SAD efficiency studies were performed with the tetragonal form of thermolysin, a 316 residue protein with a predicted Bijvoet ratio of ∼1% for an X-ray wavelength of 1.54 Å. Here we investigate different cooling methods for several different protein crystals. We find that as long as ice formation is prevented and care is taken to limit damaging dehydration effects, gas stream cooling yields lower mosaicity than more rapid cooling methods (plunge cooling and hyperquenching). To assess the impact of the cooling method at the individual protein level, structures were determined of normal plunge cooled and gas stream cooled tetragonal thermolysin.

For gas stream cooling, we employed a vial mounting procedure to transfer the crystal directly to the cold gas stream rather than moving through the low-humidity ambient air. For the nine crystal/cryoprotectant combinations tested here, gas stream cooling at 100 K using the vial mounting approach yielded lower mosaicity than normal plunge cooling into liquid nitro­gen at 77 K. For the subset of crystals tested, the anomalous signal from gas stream cooling was comparable to or stronger than that from plunge cooling. Gas stream cooling yielded a stronger anomalous signal and SAD structures could be determined more efficiently (i.e. with lower redundancy data) than with plunge cooling. The cryoprotectant used was 50% xylose, which produces the smallest cell volume differences between plunge and gas stream cooling (here a 0.07% volume difference). The differences between the refined protein structures are subtle. The Cα root-mean-square deviation (RMSD) is 0.05 Å, and the hinge bending angle between the two structures is 0.2°. o electron density maps are for small shifts of bound metal ions probably associated with the slight non-isomorphism between the two crystals. Both structures have the same 33 residues built with alternative side chain conformations, whose occupancies are highly correlated, with the largest occupancy difference being 0.1. The second cluster (181, 182 and 183) forms a part of a turn at the end of a helix and includes an interaction with a bound cation. These three residues are modeled with multiple conformations, including a peptide flip of Lys182 away from the RT configuration, which is modeled with occupancies of 0.33 and 0.26 in the plunge cooled and gas stream cooled cases, respectively. There is thus very little evidence in this particular case that faster cooling via plunging into liquid nitro­gen changes conformational ensembles present at LT compared with gas stream cooling.

> ITGTSTVGVGRGVLGDQKNINTTYSTYYYLQDNTRGNGIFTYDAKYRTTLPGSLWADADNQFFASYDAPAVDAHYYAGVTYDYYKNVHNRLSYDGNNAAIRSSVHYSQGYNNAFWNGSQMVYGDGDGQTFIPLSGGIDVVAHELTHAVTDYTAGLIYQNESGAINEAISDIFGTLVEFYANKNPDWEIGEDVYTPGISGDSLRSMSDPAKYGDPDHYSKRYTGTQDNGGVHINSGIINKAAYLISQGGTHYGVSVVGIGRDKLGKIFYRALTQYLTPTSNFSQLRAAAVQSATDLYGSTSQEVASVKQAFDAVGVK> MALNRVPSRVLPFAVSGVYVHPRNACRLPAAAAVSSVPSSVSAFSSRTNFLSRSSSAVMSHPCAATARHFSFAIPPANAAA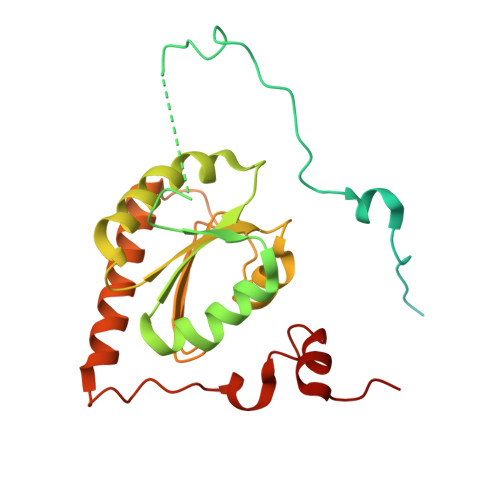LADPLPATPTPPPVFEAVSSASSGIASGTNALKNVEEVSTMERYEAAVYEESFKKPIVCLFFARFSLQSKVLLQPFLDFAASASNNATFFLIDCDRVPRAAYHARVENVPSLVVMKGDDAFRQTITDSVGVKTAGDLIQEARSALDQVLRLDQQEGGTKLQPGVSSYTHHIGVDNLNVYRKGWPVA>SMDLK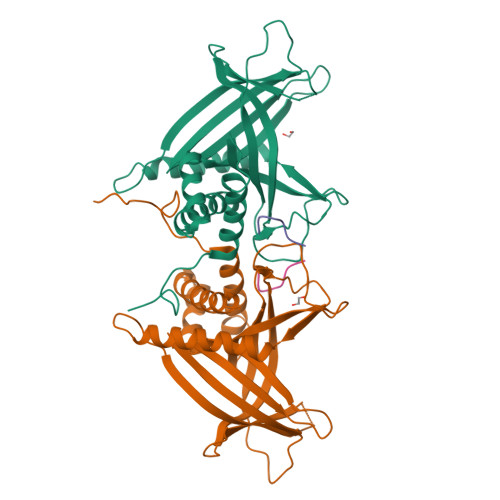GLLHEENELPSIEKRKIDENAVEHDKVERKRTKSVAVPKIEMNFLNKPIVPDTTKVISNFLTHYLITEPVEHVEIEAKLGTLIDLETQNRFEFPVMNETILNPEFNLRTRFESDMTASEHKYLNEFLNQAFRDSQKPGRLPFAYKHTKQVDLFYETEDNSRDKIRVSKNQSDNQVLACVKKRRVADLFLYCPNDAFDIRISISDELPVSMPSGNQQPSLTRLKDRVGYVHQEIKIDLTKTTQNDPVYDTTERHELEVEFGNIADLRDRAQKAKDGMEAPLFRRVQLFMDNVRILRREHS[4x];>[4x]TPAWNSGSRTPAWNSGSK>GAMGDGQSNGEAKVKKIEFSEFTVKIKNKNNSNNWADLGDLVVRKEEDGIETGLNVGKGDSDTFAGYTATFFSLEESEVNNFIKAMTEGGSFKTSLYYGYKDEQSNANGIQNKEIITKIEKIDDFEY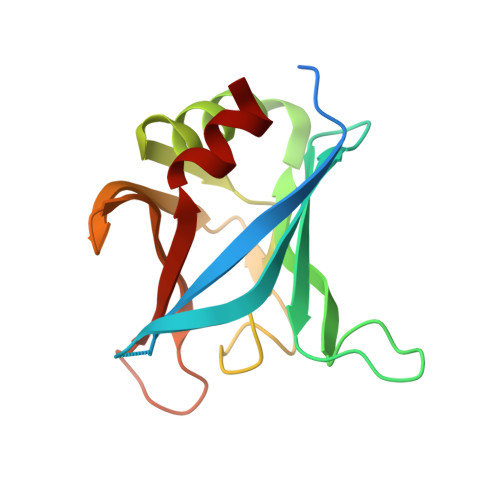ITFLGDKIKDSGDKVVEYAILLEDLKKNLK[2x]>[2x]GAHRGRVTRRNIIWHELIGLRVRIVGSTHPAFVGIEGYVIDETRNMLVIA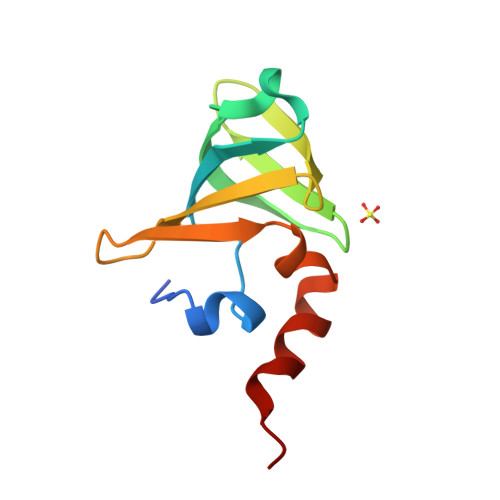GDRIWKVPKDVSIFEFEADDGTKIKIPGERLVGRPEMRLKKRWKKW>SMIMEIPAIKALSRYAQWVIWKKERDTKIPYNPNNGKKASSTDPLAWGDIDEAQAGLVRYGANGLGFVLTKSDPFVFIDLDHVLDENKRVKCEWARQLLKEIKSYTEISPSGDGLHVVVSGKLPDYIKHKTKFDDGSALEVYESGRYMTITGEVFDGRDDIKELDLSILGEFAEHKIETKNAPVQIESATTLDDEAIIDLMKRKGQWPDAPKDGDDWSSLDMSFANRLAFWCGKDIERMDRIFRQSPLMRQKWDRPTAGSTYGR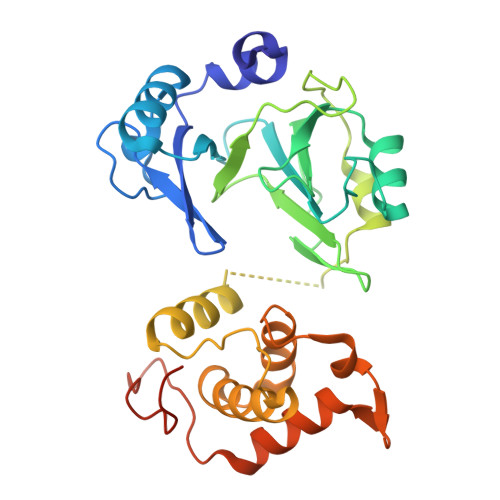ITLKKACDFVDSVYDPALRNESDCPFEPYNEEGGPRNDKEEK[2x]In this context, we recently proposed a lanthanide-based molecule, named the crystallophore (Tb-Xo4). Tb-Xo4 is a cationic complex with nucleating and phasing properties. In particular, we show that Tb-Xo4 may provide different crystal forms of a single protein and correct the often-encountered defects in crystalline order that may result in low-resolution data as well as twinning. We prove that, beyond these crystallization properties, Tb-Xo4 is one of the most efficient phasing tools compatible with serial crystallography approaches.

We performed two SAD phasings by merging several data sets obtained through the MeshAndCollect approach using protease 1 and pb9. P. horikoshii protease 1 (PhP1) crystallization was performed in sodium malonate pH 5.5. Crystals with dimensions ranging from 10 × 10 × 10 µm to 30 × 30 × 30 µm were used. Data were collected on four different mesh loops corresponding to four different crystallization drops, leading to 81 sub-data sets. Among them 27 were selected and merged by HCA using ccCluster with a distance definition based on the correlation between intensities and with a coefficient linkage threshold value of 0.3 [Fig. 1(a)], resulting in statistics indicated in Table 1. Despite the soaking in the concentrated solution of Tb-Xo4, half of the crystals, coming from four different supports, were sufficiently isomorphous to allow the merging of their respective data sets. For both presented examples, even with soaking of the crystals in a solution containing 100 mM Tb-Xo4, the level of isomorphism between the crystals was sufficiently preserved and kept sufficiently high to derive useful phases.

>MKVLFLTANEFEDVELIYPYHRLKEEGHAVYIASFERGTITGKHGYSVKVDLTFDKVNPAEFDALVLPGGRAPERVRLNAKAVSIARKMFSEGKPVASICHGPQILISAGVLRGRKGTSYPGIKDDMINAGVEWVDAEVVVDGNWVSSRVPADLYAWMREFVKLLK[3x]ethyl 3,4,5-trihydroxybenzoate | C9 H10 O5 | 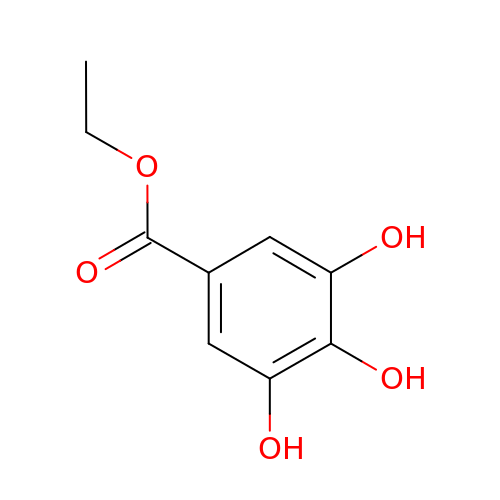VFPFQHQNJCMNBZ-UHFFFAOYSA-N>[2x]MGSDKIHHHHHHMKVSEFDYELPPELIAQEPVEPRDASRLMVLHRKTQRIEHRIFREIIEYLEPGDLLVLNVSKVIPARLYARKKTGASIEILLIERLEEGIWKCLVRPGQ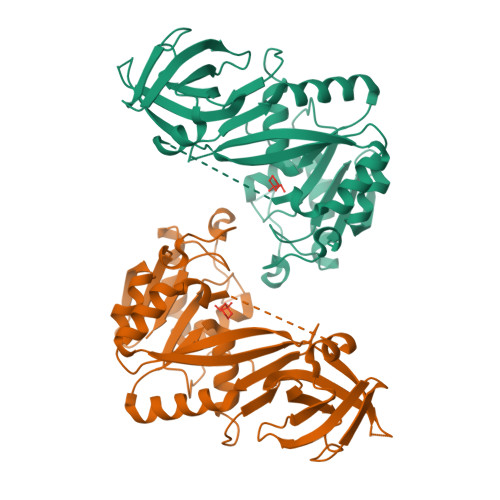KVKKGTELVIDEDLSAVCLGRGEDGTRILKFQPQDDRLIFEKGRTPLPPYIKNEVPLERYQTVYAKEEGSVAAPTAGLHFTPELIEKLKKKGVQFAEVVLHVGIGTFRPVKVEEVEKHKMHEEFYQVPKETVRKLRETRERGNRIVAVGTTTVRTLETIARLPEQEEYVGKTDLFIYPPFEFKLVDALVTNFHLPRSTLLMLVAAFAGKDFVMEAYREAVKRRYRFFSFGDAMLIL> MEFMRVLLIAGGVSPEHEVSLLSAEGVLRHIPFPTDLAVIAQDGRWLLGEKALTALEAKAAPEGEHPFPPPLSWERYDVVFPLLHGRFGEDGTVQGFLELLGKPYVGAGVAASALCMDKDLSKRVLAQAGVPVVPWVAVRKGEPPVVPFDPP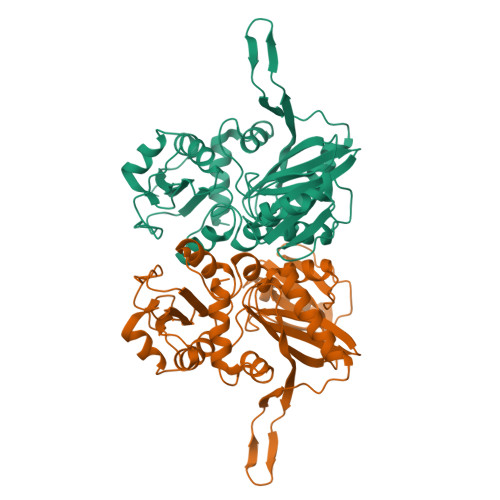FFVKPANTGSSVGISRVERFQDLEAALALAFRYDEKAVVEKALSPVRELEVGVLGNVFGEASPVGEVRYEAPFYDYETKYTPGRAELLIPAPLDPGTQETVQELALKAYKVLGVRGMARVDFFLAEGELYLNELNTIPGFTPTSMYPRLFEAGGVAYPELLRRLVELALT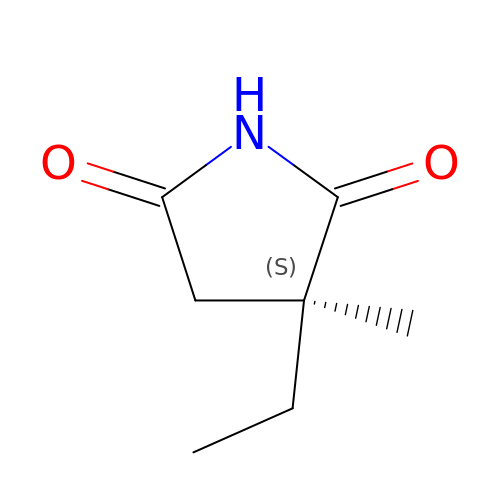(3~{S})-3-ethyl-3-methyl-pyrrolidine-2,5-dione | C7 H11 N O2 | HAPOVYFOVVWLRS-ZETCQYMHSA-N>[2x]MDHYLYAINPNGKLKWKFETGGSVHSSPAIGQDGTIYVGSND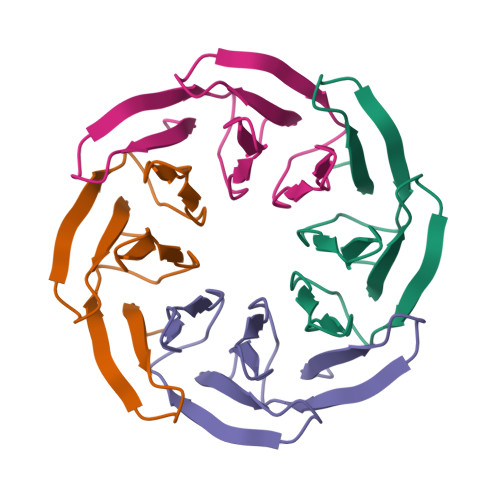HYLYAINPNGKLKWKFETGGSVHSSPAIGQDGTIYVGSN> DADLAKKNNCIACHQVETKVVGPALKDIAAKYADKDDAATYLAGKIKGG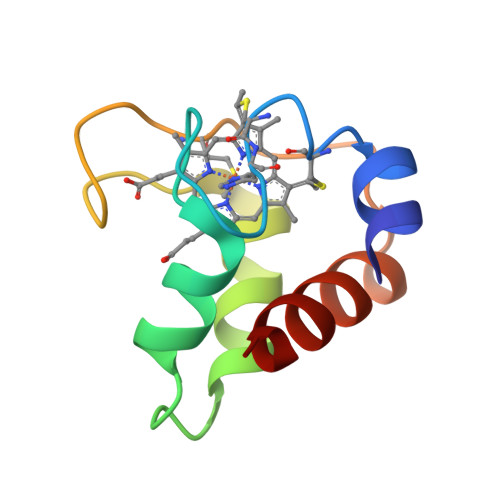SSGVWGQIPMPPNVNVSDADAKALADWILTLK> MSIWKEAKDASGRIYYYNTLTKKSTWEKPKELISQEELLLRENGWKAAKTADGKVYYYNPTTRETSWTIPAFEKKVEPIAEQKHDTVSHAQVNGNRIALTAGEKQEPGRTINEEESQYANNSKLLNVRRRTKEEAEKEFITMLKENQVDSTWSFSRIISELGTRDPRYWMVDDDPLWKKEMFEKYLSNRSADQLLKEHNETSKFKEAFQKMLQNNSHIKYYTRWPTAKRLIADEPIYKHSVVNEKTKRQTFQDYIDTLIDTQKESKKKLKTQALKELREYLNGIITTSSSETFITWQQLLNHYVFDKSKRYMANRHFKVLTHEDVLNEYLKIVNTIENDLQNKLNELRLRNYTRDRIARDNFKSLLREVPIKIKANTRWSDIYPHIKSDPRFLHMLGRNGSSCLDLFLDFVDEQRMYIFAQRSIAQQTLIDQNFEWNDADSDEITKQNIEK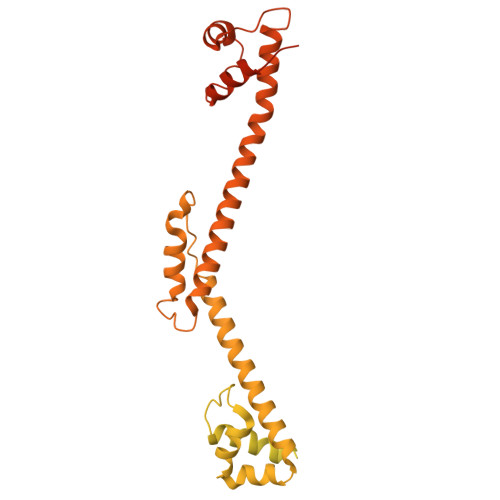VLENDRKFDKVDKEDISLIVDGLIKQRNEKIQQKLQNERRILEQKKHYFWLLLQRTYTKTGKPKPSTWDLASKELGESLEYKALGDEDNIRRQIFEDFKPESSAPTAESATANLTLTASKKRHLTPAVELDY>[9x]SADVAGAVIDGAGLGFDVLKTVLEALGNVKRKIAVGIDN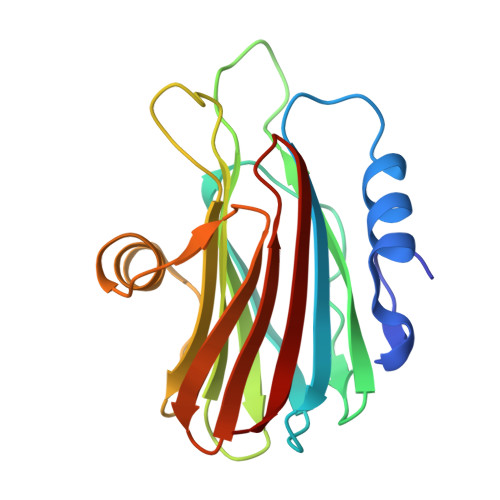ESGKTWTAMNTYFRSGTSDIVLPHKVAHGKALLYNGQKNRGPVATGVVGVIAYSMSDGNTLAVLFSVPYDYNWYSNWWNVRVYKGQKRADQRMYEELYYHRSPFRGDNGWHSRGLGYGLKSRGFMNSSGHAILEIHVTKA> MTALFLHILWSISYIIINILYIFLSLLLSNNNEKIKQYNSNYFIKILLVLFYNKNLSFYKNLLSEDEISKIEFERLKNYPTLVLIHSNLNKLEKRNKIINSFINFKTKYRFYKFISTNFNLQTIIKNCNDKIIFSTLLYIVNLNYSFFYKTIKNTDLIVYLLANKFSILNDNIIVSKFNISKFNDYIKYINNTNSIDTYLENQIILGLN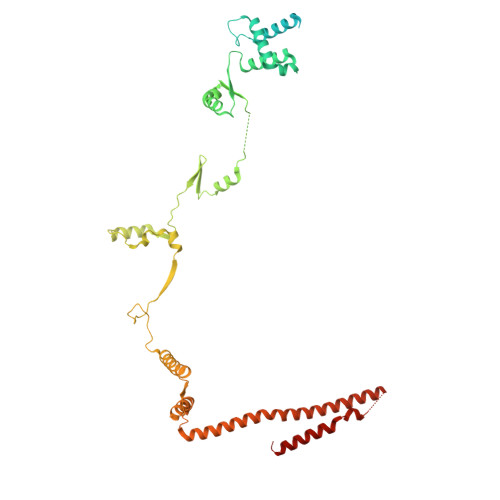NNTNSNITKNINTKLLNSYSNLKNLVNITNNTFYLKKINDNYNTVINSEFLTYLKSNYKISFSASNIVKYLSDKSVNNSVILYLRKNKIFNKSRYSRNRQTYRTGAYWCLYVNIIAVVAFYFWFYKFTMNFGYLWWLLYSLILSFFFSRALKHRFYNPLNVMTEFKNGFMWFIIILINIFKPLLKLLENNYINLYNHLVIKYYQSFICNTLINKKKLEFNYILSSFKFIKELNNIIIISLNKLF> QPNVDMGFEAAVAKKVVVPITFMVPNRPSGLTQSALLVTGRTFLINEHTWSNPSWTSFTIRGEVHTRDEPFQTVHFTHHGIPTDLMMVRLGPGNSFPNNLDKFGLDQMPARNSRVVGVSSSYGNFFFSGNFLGFVDSITSEQGTYARLFRYRVTTYKGWAGSALVCEAGGVRRIIGLHSAGAAGIGAGTYI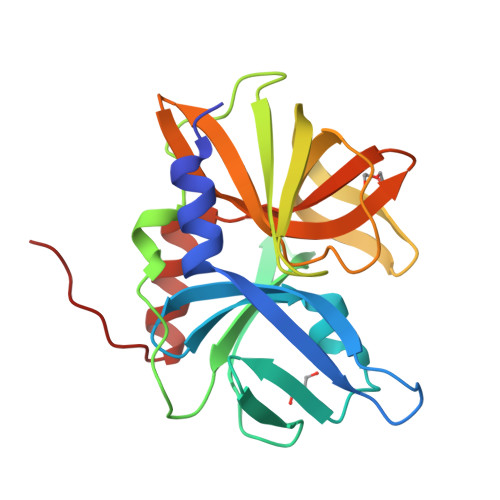SKLGLIKALKHLGEPLATMQ> ATDTGGYAATAGGNVTGAVSKTATSMQDIVNIIDAARLDANGKKVKGGAYPLVITYTGNEDSLINAAAANICGQWSKDPRGVEIKEFTKGITIIGANGSSANFGIWIKKSSDVVVQNMRIGYLPGGAKDGDMIRVDDSPNVWVDHNELFAANHECDGTPDNDTTFESAVDIKGASNTVTVSYNYIHGVKKVGLDGSSSSDTGRNITYHHNYYNDVNAKLPLQRGGLVHA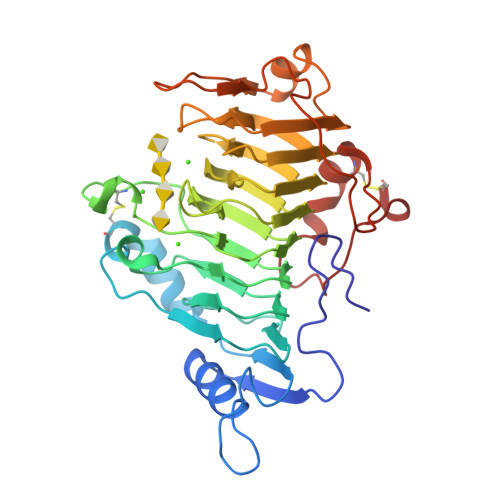YNNLYTNITGSGLNVRQNGQALIENNWFEKAINPVTSRYDGKNFGTWVLKGNNITKPADFSTYSITWTADTKPYVNADSWTSTGTFPTVAYNYSPVSAQCVKDKLPGYAGVGKNLATLTSTACK>GPQQEDEKMILSFDKAIQYMSKRKIGALITIERHTGLDEYIETGIALDADITGELLINIFIPNTPLHDGAVIVKEGKIAVASAYLPLSESMLIPKEFGTRHR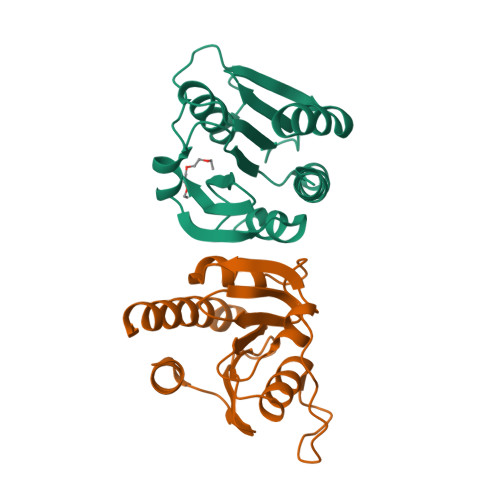AAVGISEVSDAITIVVSEETGDVSITLDNELMAGLSQQEYLAILRRELI[2x]>[2x]MSLGVTQASAQWGVKASFQNYIRGSIANGSWTLNGVGFDNQQFQFSGNSGAVDAENKTGSINFPGSIHFTGAGGILDMQIANIEISFNGNS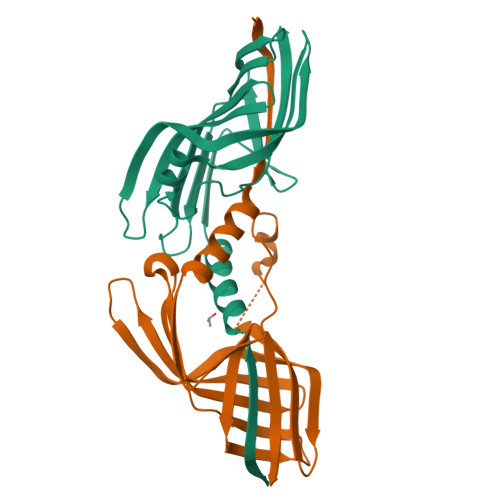GELIADVVSSDMDGNSTNYGRTVVGTLNFSALNVSATEASGSASVSLSQSGSQAFADFYTPGTQLDPISFSATLGGLEHHHHHH> AMDLRVGRKFRIGRKIGSGSFGDIYHGTNLISGEEVAIRLESIRSRHPQLDYESRVYRYLSGGVGIPFIRWFGREGEYNAMVIDLLGPSLEDLFNYCHRRFSFKTVIMLALQMFCRIQYIHGRSFIHRDIKPDNFLMGVGRRGSTVHVIDFGLS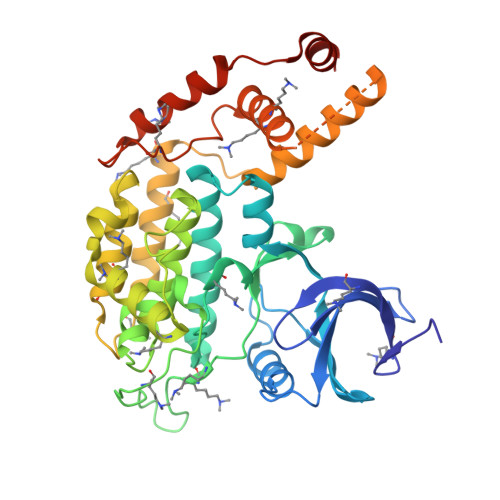KKYRDFNTHRHIPYRENKSLTGTARYASVNTHLGIEQSRRDDLESLGYVLIYFCKGSLPWQGLKATTKKQKYDRIMEKKLNVSVETLCSGLPLEFQEYMAYCKNLKFDEKPDYLFLARLFKDLSIKLEYHNDHLFDWTMLRYTKAMVEKQRDLLIEKGDLNANSNAASASNSTDNKSETFNKIKLLAMKKFPTHFHYYKNEDKHNPSPEEIKQQTILNNNAASSLPEELLNALDKGMENLR>CTTNYVMTTKNGQTI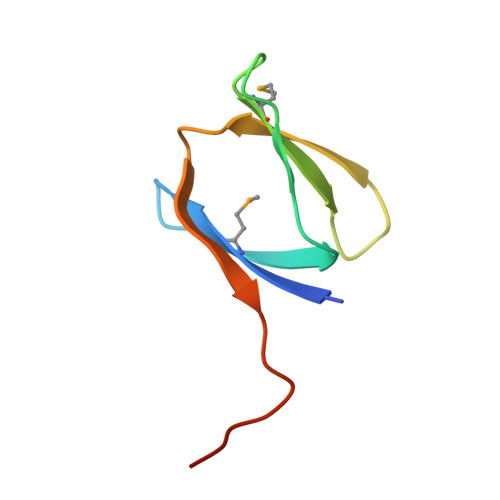VTQGKPQLDKETGMTSYTDQEGNQREINSNDVAQLIKADLEHHHHHH[3x]>MGSKSFLTEQQIKILRLRARGLKQSEIAELLGTSRANISILERRALEKIEKARNTITIWEQINSKISVEVRKGEDIFTVPDKLFKKADELQIKVPYSTAEIIAFLVEHAPISDRIAKRDFTLFLDARDRLRISECLLEEFDEIGKQHH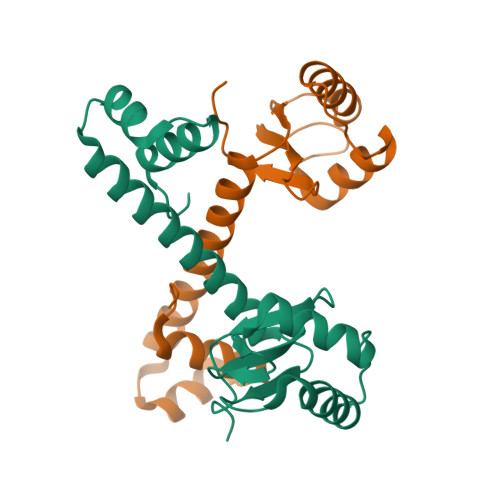HHHH[2x]> ADLGTENLYFQSMKPSPEEAQLWSEAFDELLASKYGLAAFRAFLKSEFCEENIEFWLACEDFKKTKSPQKLS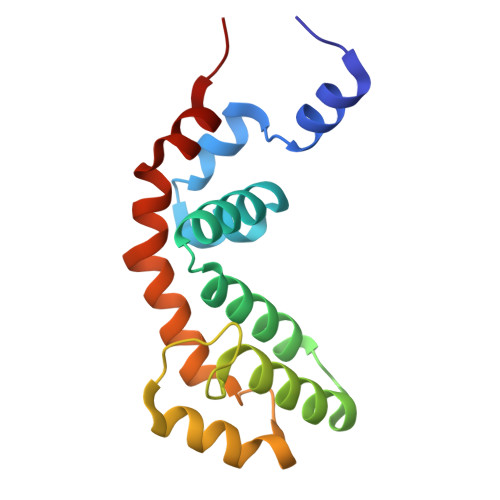SKARKIYTDFIEKEAPKEINIDFQTKTLIAQNIQEATSGCFTTAQKRVYSLMENNSYPRFLESEFYQDLCKKPQ>GSGPAFESYESMELACPAERSGHVAVSDGRHMFVWGGYKSNQVRGLYDFYLPREELWIYNMETGRWKKINTEGDVPPSMSGSCAVCVDRVLYLFGGHHSRGNTNKFYMLDSRSTDRVLQWERIDCQGIPPSSKDKLGVWVYKNKLIFFGGYGYLPEDKVLGTFEFDETSFWNSSHPRGWNDHVHILDTETFTWSQPITTGKAPSPRAAHACATVGNRGFVFGGRYRDARMNDLHYLNLDTWEWNELIPQGICPVGRSWHSLTPVSSDHLFLFGGFTTDKQPLSDAWTYCISKNEWIQFNHPYTEKPRLWHTACASDEGEVIVFGGCANNLLVHHRAAHSNEILIFSVQP[2x]

CRL2KLHDC2 has been proposed as an attractive additional E3 ligase handle for targeted protein degradation. Specifically, KLHDC2 recognizes substrates possessing a Gly-Gly C-terminal degron (C-degron) sequence. First, crystal structures showed KLHDC2 binds substrate C-termini in a well-defined pocket lined by aromatic residues available to engage a ligand. Ligands were identified that engage the C-degron binding site in KLHDC2, subjected to structure-based improvement, and linked to JQ1 for BET-family neo-substrate recruitment.

We therefore tested if expanding the phenyl group into naphthyl or bi-aryl analogs, which could potentially better fill this pocket, would improve binding. Amongst the various naphthyl analogs tested, SJ46411 exhibited excellent activity with a Kd of ~260 nM measured by isothermal titration calorimetry (SPR Kd = 0.5 μM, TR-FRET IC50 = 3.9 μM, ΔTm = 6.0 °C). We also note that the 2-naphthyl substitution demonstrated greater activity than the 1-naphthyl substitution (SJ46411 vs SJ46145). A co-crystal structure of SJ46411 bound to KLHDC2 confirmed the predicted stacking of the hydrophobic face of the naphthyl ring in the binding pocket. The structure further showed the di-Gly portion of the molecule allows a water-mediated bridge between the thiazole ring and acid moieties. To evaluate potential exit vectors, we compared structures of KLHDC2 bound to SJ46411 and to a di-Gly substrate peptide. This analysis revealed that linker attachment to position 8 of the naphthyl ring would generate an exit vector closely matching that of a natural substrate. The data showed a greater than two orders-of-magnitude selectivity of SJ46421 for KLHDC2 over other KLHDC-family CRLs. Consistent with this view, SJ46411 and SJ46421 alone were only able to inhibit KLHDC2 substrate ubiquitylation and largely inactive towards other the Kelch family E3 ligases.> GSQSQLSHQDLQLVKGAMAATYSALNSSKPTPQLKP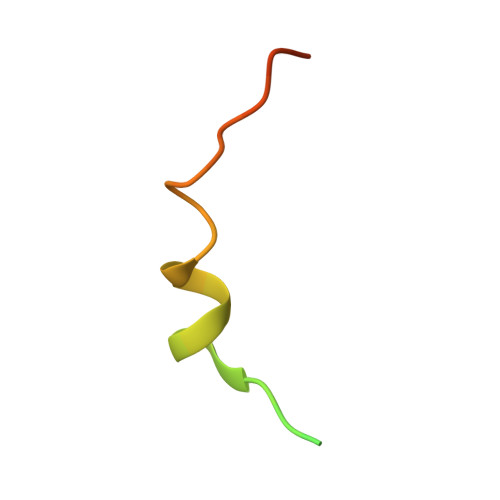IESS> MLDFTEASLKKVLTRYNVALEKALTPEEAAEELYPKDELIYPIAKAIFEGEEDDVVEGLQAAIEAGKDPIDLIDDALMVGMGVVIRLYDEGVIFLPNVMMSADAMLEGIEYCKENSGATPKTKGTVVCHVAEGDVHDIGKNIVTALLRANGYNVVDLGRDVPAEEVLAAVQKEKPIMLTGTALMTTTMYAFKEVNDMLLENGIKIPFAC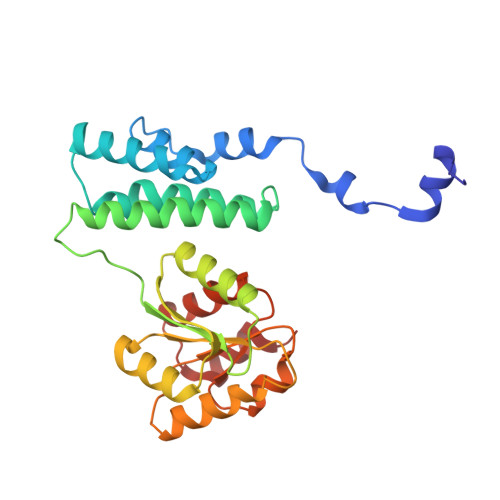GGGAVNQDFVSQFALGVYGEEAADAPKIADAIIAGTTDVTELREKFHKH>[2x]GPLGSHMSTESNDGVSETLLAWRHIDFWTSEHNPDLNATLSDPCTQ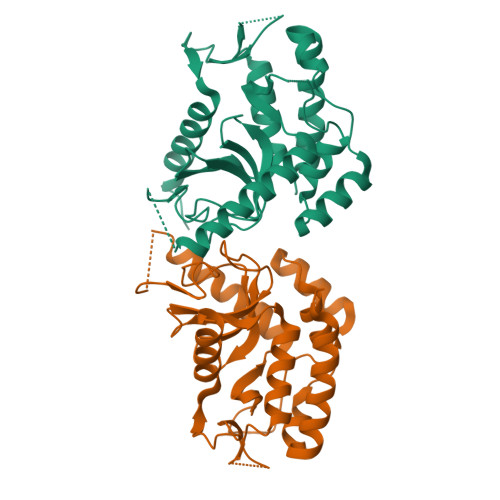NDITHAEEDLEVSFPNPVKASFKIHDGQEDLESMTGTSGLFYGFQLMTLDQVVAMTQAWRNVAKNLNKRSQQGLSHVTSTGSSSSMERLNGNKFKLPNIPDQKSIPPNAVQPVYAHPAWIPLITDNAGNHIGVDLAPGPNGKYAQIITFGRDFDTKFVIAENWGEFLLSFANDLEAGNWYLVDDNDDYFSGDGELVFRDKKSNGPIQDYFEVLKRRTWIKYQLERPHRD>MAMLTKFESRSSRAKGVAFHPTQPWILTSLHNGRIQLWDYRMGTLLDRFDGHDGPVRGIAFHPTQPIFVSGGDDYKVNVWNYKSRKLLFSLCGHMDYVRVCTFHHEYPWILSCSDDQTIRIWNWQSRNCIAILTGHSHYVMCAAFHPSEDLIVSASLDQTVRVWDISGLRMKNAAPVSMSKEDQKAQAHNSISNDLFGSADAIVKFVLEGHDRGVNWCAFHPTLPLILSAGDDRLVKLWRM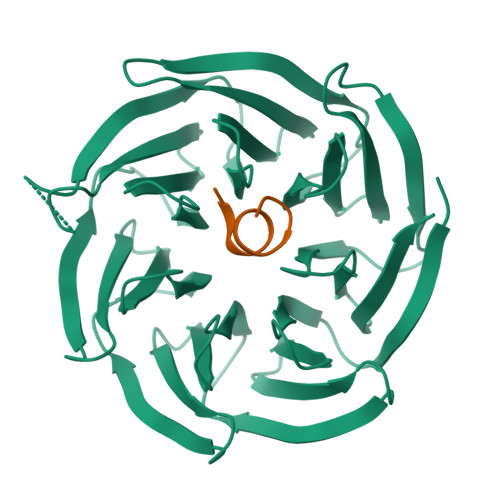TASKAWEVDTCRGHFNNVSCCLFHPHQELILSASEDKTIRVWDLNRRTAVQTFRRANDRFWFITVHPKLNLFAAAHDSGVMVFKLE[2x];>AASFIDAKKMP[2x]nonyl 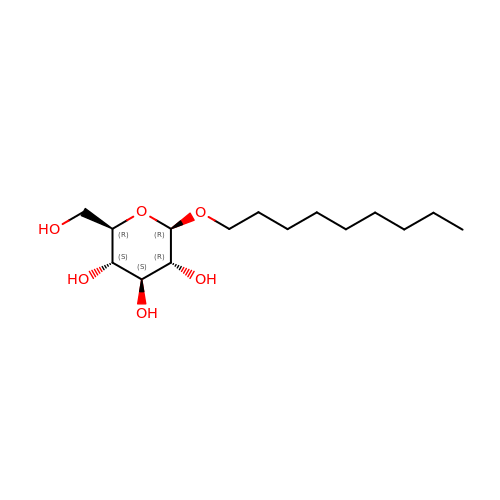beta-D-glucopyranoside | C15 H30 O6 | QFAPUKLCALRPLH-UXXRCYHCSA-N[(1S)-1-hydroxypropyl]phosphonic 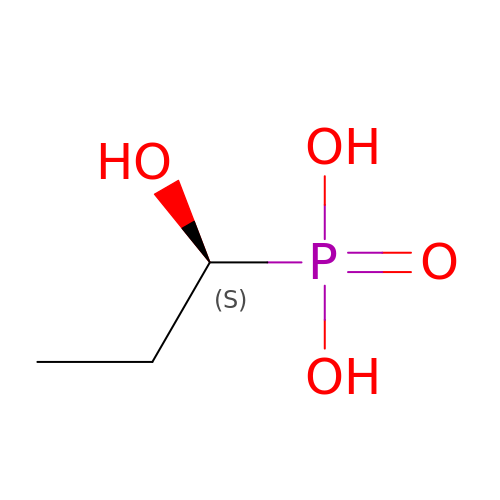acid | C3 H9 O4 P | MVIJUJBSAAUHEM-VKHMYHEASA-N>MAEEGTRSEAADAATQARQLPDSRNIFVSHRFPERQVDLGEVVMNFAEAGSPDNPALLLLPEQTG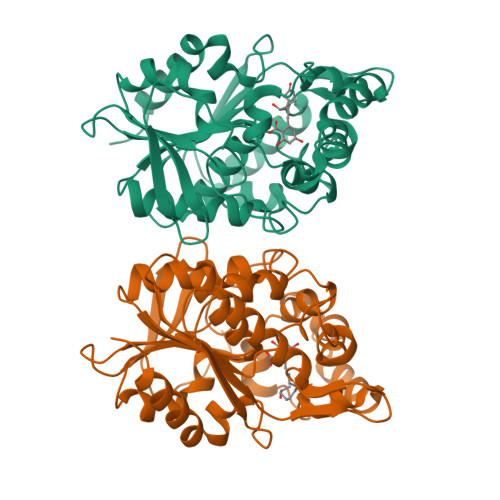SWWSYEPVMGLLAENFHVFAVDIRGQGRSTWTPRRYSLDNFGNDLVRFIALVIKRPVVVAGNSSGGLLAAWLSAYAMPGQIRAALCEDAPFFASELVPAYGHSVLQAAGPAFELYRDFLGDQWSIGDWKGFVEAAKASPAKAMQLFPTPDEAPQNLKEYDPEWGRAFFEGTVALHCPHDRMLSQVKTPILITHHARTIDPETGELLGALSDLQAEHAQDIIRSAGVRVDYQSHPDALHMMHLFDPARYAEILTSWSATLPANDHHHHHH[4x]>[4x]MSQSQRSTADWQRLDAAHHLHPFTDYGELNTKGSRIITRAEGCYLWDSDGNQILDGMAGLWCVNIGYGRKELAEVAYRQMQELPYYNNFFQCSHPPAIELSRLLSEVTPKHMNHVFFTGSGSDSNDTILRMVRYYWKLLGKPYKKVVISRENAYHGSTVAGASLSGMKAMHSHGDLPIPGIEHIEQPYHFGRAPDMDPAEFGRQAAQALERKIDEIGECNVAAFIAEPIQGAGGVIIPPDSYWPEIKRICAERDILLIVDEVITGFGRLGTWFGSQYYDLQPDLMPIAKGLSSGYMPIGGVMVSDRVAKVVIEEGGEFFHGYTYSGHPVAAAVAAENIRIMRDEGIIERAGAEIAPYLQARWRELGEHPLVGEARGVGMVAALELVKSKQPLERFEEPGKVGSLCRDLSVKNGLVMRAVGGTMIISPPLVLSREQVDELIDKARRTLDETHKAIGGALEHHHHHH

Herein we present the development of a PluriZyme, TR2E2, with efficient native transaminase (k cat: 69.49±1.77 min−1) and artificial esterase (k cat: 3908–0.41 min−1) activities integrated into a single scaffold, and evaluate its utility in a cascade reaction. The reaction proceeds through the conversion of the β‐keto ester into the β‐keto acid at the hydrolytic site and subsequently into the β‐amino acid (e.e. >99 %) at the transaminase site. In addition, we report the crystal structures of the TR2 enzyme and the newly designed TR2E2 PluriZyme. It presents the typical type I fold of class III ω‐TA observed in known structures present in the PDB database, and it contains the characteristic pyridoxal‐5′‐phosphate (PLP)‐binding domain composed of β‐sheets and the catalytic base Lys289.

Additionally, we succeeded in growing crystals and solving the structure of TR2E2 bound to the PLP cofactor (resolution of 3.5 Å) and in complex with the ethanolamine O‐sulfate (EOS) inhibitor (resolution of 3.6 Å), located in the transaminase catalytic center. The artificial esterase catalytic triad was observed in the TR2E2 crystal structures and is composed of Ser172 and His173 of chain A (magenta) and Glu317 of chain B (green); similar to the transaminase's active site, the esterase site is composed of a functional protein dimer. Notably, the distance between both active sites is ≈20 Å, with the esterase site being more solvent‐exposed and located at the beginning of the tunnel and the transaminase site being more buried in the protein structure. When the residues Ser172 and His173 were replaced with Ala, the activity was completely abolished. Thus, the A172S and Q173H mutations in TR2E2 (located at site G in Figure 2) do not exert a deleterious effect on the original transaminase activity and, importantly, confer esterase activity.The first documented single-component Trp-FDH is AetF from cyanobacterium *Aetokthonos hydrillicola*, which catalyzes consecutively bromination on C5 and then C7 of Trp to generate 5,7-di-Br-Trp. More recently, a class of “single-component” FDHs has been identified. These enzymes fuse pyridine nucleotide-dependent flavin reductase and FDH on the same polypeptide chain, an advantageous feature in the application aspect relative to canonical FDHs owing to the omission of including a flavin reductase. The action of FDHs requires the reduced flavin and molecular oxygen to generate hydroperoxyl flavin intermediate, which oxidizes a halide ion to form a halogenating reagent hypohalous acid (HOX). The flipping allows the carbon-to-be-halogenated to be oriented toward the catalytic residue K258 and within the hydrogen bond distance to the putative general base E200, such that the halogenation site on two substrates is switched from C5 to C7.

We thus focused on modifying M216, F372 and L183 and eventually obtained recombinant proteins of triple variants including AI-L183F, AI-M216Y and AI-M216W and had their catalytic activity tested. AI-L183F, termed AetF-AIF hereinafter, shows higher production of 5-Br-Trp compared with wild type AetF (271 ± 7.7 %). Despite the 5-Br-Trp production level of AetF-AIF is slightly lower than AetF-AI (271 ± 7.7 % vs. 306.7 ± 6.9 %) (**[Fig fig2]**), this variant produces no detectable di-brominated product from 5-Br-Trp in reaction incubated as long as 8 hrs (**[Fig fig2] and Fig. S2**). Therefore, AetF-AIF was tentatively defined as a C5 Trp-FDH, which was subjected to the subsequent investigations. As shown in **[Table tbl2]**, AetF-AIF exhibits higher *K*_M_ and *k*_cat_ against Trp compared with the wild type enzyme, suggesting that the triple mutations render AetF higher catalytic rate and lower Trp-binding capacity. Structural investigations indicate that Trp adopts the same binding pose in wild type enzyme and AetF-AIF (**[Fig fig3]**). We solved the complex structure of AetF-AIF and Trp and found that the bulge that accommodates the Br on the 5-Br-Trp is missing AetF-AIF (**[Table tbl1] and [Fig fig3]**). Altogether, we conclude that blocking the space near C5 in 5-Br-Trp in the AetF/5-Br-Trp in addition to preventing the flipping of the substrate is required to achieve complete elimination of C7-halogenation activity of AetF-AIF. In comparison, variant AetF-AIF shows highly specific regioselectivity and comparable activity to the wild type enzyme.

> MLEVCIIGFGFSAIPLVRELARTQTEFQIISAESGSVWDRLSESGRLDFSLVSSFQTSFYSFDLVRDYEKDYYPTAKQFYEMHERWRSVYEEKIIRDFVTKIENFKDYSLISTRSGKTYEAKHVVLATGFDRLMNTFLSNFDNHVSNKTFVFDTMGDSANLLIAKLIPNNNKIILRTNGFTAFDQEVQVLGKPFTLDQLESPNFRYVSSELYDRLMMSPIYPRTVNPAVSYNQFPLIRRDFSWVDSKSSPPNGLIAIKYWPIDQYYYHFNDDLENYISKGYLLNDIAMWLHTGKVILVPSDTPINFDKKTITYAGIERSFHQYVKGDAEQPRLPTILINGETPFEYLYRDTFMGVIPQRLNNIYFLGYTRPFTGGLANITEMQSLFIHKLITQPQFHQKIHQNLSKRITAYNQHYYGAAKPRKHDHTVPFGFYTEDIARLIGIHYQPNECRSVRDLLFYYAFPNNAFKYRLKGEYAVDGVDELIQKVNDKHDHYAQVFVQALSIRNMNSDEAAEWDHSARRFAFNDMRHKEGYRAFLDTYLKAYRQVENISVDDTVVDEEWNFMVKEACQVRDKVAPNIEEKTHYSKDEDVNKGIRLILSILDSDISSLPDSNGSRGSGNLKEGDRLCKFEAQSIEFIRRLLQPKNYELLFIRESTVSPGSHRHGETA>MKRQGKRPSKNLKARCSRKALHVNFKDMGWDDWIIAPLEYEAFHCEGLCEFPLRSHLEPTNHAVIQTLMNSMDPESTPPTCCVPTRLSPISILFIDSANNVVKKDYEDMVVESCGCR[2x];>[2x]ETGQCRIQKCTTDFVSLTSHLNSAVDGFDSEFCKALRAYAGCTQRTSKACRGNLVYHSAVLGISDLMSQRNCSKDGPTSSTNPEVTHGTKHHHHHH

Repulsive guidance molecules (RGMs) are cell surface proteins that control processes ranging from brain development to iron metabolism. RGMs can bind to the cell guidance receptor Neogenin (NEO1) and act as coreceptors for the bone morphogenetic proteins (BMPs). Structural analysis of RGMs and their complexes with NEO1 and BMP2 revealed a common RGM architecture comprising an N-terminal domain (RGMND) essential for BMP binding and a C-terminal domain (RGMCD) sufficient for NEO1 binding. Here, we determined high-resolution structures of all three human RGMs in complex with the BMP ligand growth differentiation factor 5 (GDF5) and the ternary complex of GDF5 with RGM and NEO1.

To characterize the RGM–GDF5 interactions, we determined the crystal structure of RGMBND in complex with GDF5 at 1.7 Å resolution. In the complex, the disulfide-linked GDF5 dimer binds two RGMBND molecules that are related by a noncrystallographic pseudo twofold axis (RMSD of 0.21 Å for 143 equivalent Cα atoms of the 1:1 RGMB:GDF5 complexes). RGMBND forms a bundle of three α-helices stabilized by three disulfide bonds. It binds to the finger region of GDF5 and interacts with both GDF5 molecules of the dimer. The RGMBND–GDF5 interface comprises mixed charged and hydrophobic interactions (containing 116 nonbonded contacts and 5 hydrogen bonds) mediated by 20 residues from each binding partner and buries a total surface area of 1,929 Å2. The side-chain of RGMB Leu103 inserts into the hydrophobic pocket on GDF5 formed by Trp414, Trp417, Ile449, Tyr490, and Met493 and is shielded by a hydrogen bond formed by RGMB Gly101 (“RGD-loop”) and GDF5 Tyr490. A major interface is formed by the side-chain of RGMB His106 that stacks onto GDF5 Trp417. This π–π stacking is shielded from the solvent by RGMB Arg100. Our 1.7 Å crystal structure allowed us to identify a network of well-ordered water molecules contributing to the RGMB–GDF5 interactions. The side-chain of RGMB His106 forms a hydrogen bond with the amide of Gly101 from the “RGD-loop” and a water molecule that extends a hydrophilic network to Tyr105, Trp414, and Asp416 of GDF5.>HGGEAHMVPMDKTLKEFGADVQWDDYAQLFTLIKDGAYVKVKPGAQTAIVNGQPLALQVPVVMKDNKAWVSDTFINDVFQSGLDQTFQVEKRPHPLNALTADEIKQAVEIVKASADFKPNTRFTEISLLPPDKEAVWAFALENKPVDQPRKADVIMLDGKHIIEAVVDLQNNKLLSWQPIKDAHGMVLLDDFASVQNIINNSEEFAAAVKKRGITDAKKVITTPLTVGYFDGKDGLKQDARLLKVISYLDVGDGNYWAHPIENLVAVVDLEQKKIVKIEEGPVVPVPMTARPFDGRDRVAPAVKPMQIIEPEGKNYTITGDMIHWRNWDFHLSMNSRVGPMISTVTYNDNGTKRKVMYEGSLGGMIVPYGDPDIGWYFKAYLDSGDYGMGTLTSPIARGKDAPSNAVLLNETIADYTGVPMEIPRAIAVFERYAGPEYKHQEMGQPNVSTERRELVVRWISTVGNYDYIFDWIFHENGTIGIDAGATGIEAVKGVKAKTMHDETAKDDTRYGTLIDHNIV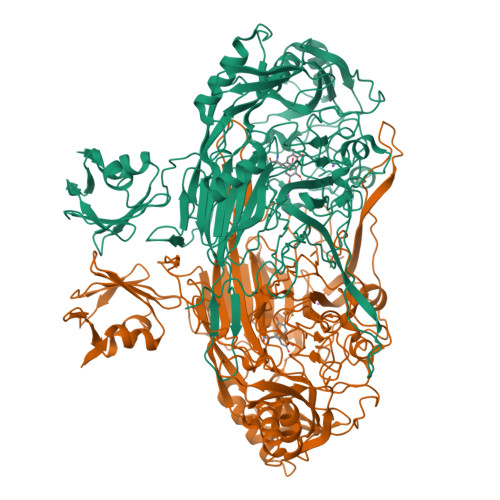GTTHQHIYNFRLDLDVDGENNSLVAMDPVVKPNTAGGPRTSTMQVNQYNIGNEQDAAQKFDPGTIRLLSNPNKENRMGNPVSYQIIPYAGGTHPVAKGAQFAPDEWIYHRLSFMDKQLWVTRYHPGERFPEGKYPNRSTHDTGLGQYSKDNESLDNTDAVVWMTTGTTHVARAEEWPIMPTEWVHTLLKPWNFFDETPTLGALKKDK[2x]F17 and F18 fimbriae are wire-like structures expressed on the surface of enterotoxigenic and septicemic Escherichia coli (ETEC) strains that secrete toxins causing diarrhea in infantile livestock. F17, F18 and type-1 fimbriae are assembled by the chaperone/usher biogenesis pathway and comprise a few thousand copies of a major pilin (F17A, FedA and FimA respectively), several minor pilin proteins and a single two-domain adhesin (TDA) at the tip (F17G, FedF and FimH, respectively). The N-terminal domain of TDAs is a lectin domain, also called receptor-binding domain, because it mediates adherence of fimbriated bacteria to glycoconjugate receptors on host epithelial linings. Amino acid sequence and crystal structure analyses of the lectin domains of F17G, FedF and FimH elucidate a previously unacknowledged basis for strain-dependent glycan binding profiles of E. coli fimbrial adhesins, one that is driven by electrostatic interactions.

Surface Plasmon Resonance (SPR) interaction studies using a newly synthesized GlcNAcβ1-xGal series (x being 2, 3, 4 or 6) and F17G crystal structures in complex with these disaccharides provide insight in the structural basis of the variant-specific binding profiles. In each of these complexes, a terminal, non-reducing GlcNAc occupies the primary binding pocket in the same orientation as observed in the initial F17aG structure with GlcNAc. F17aG is indeed highly positively charged, with three more lysines and one more arginine than F17bG. Near the non-reducing end of the disaccharide, Arg93 (purple) is bridging the GlcNAc residue and the sulfate ion S4, whereas variable residue Asn90 (cyan) of F17bG, substituted for Lys90 in F17aG, is bridging the O4 hydroxyl of the reducing galactose and the sulfate ion S4. The majority of the amino acid variations involve arginine or lysine, which consistently lead to either an introduction or a removal of a positive charge.

> AVSFIGSTENDVGPSLGSYSRTHAMDNLPFVYDTRNKIGYQNANVWHISKGFCVGLDGKVDLPVVGSLDGQSIYGLTEEVGLLIWMGDTKYSRGTAMSGNSWENVFSGWCVGANTASTQGLSVRVTPVILKRNSSARYSVQKTSIGSIRMRPYNGSSAGSVQTTVNFSLNPFTLNDT> MASSNVTL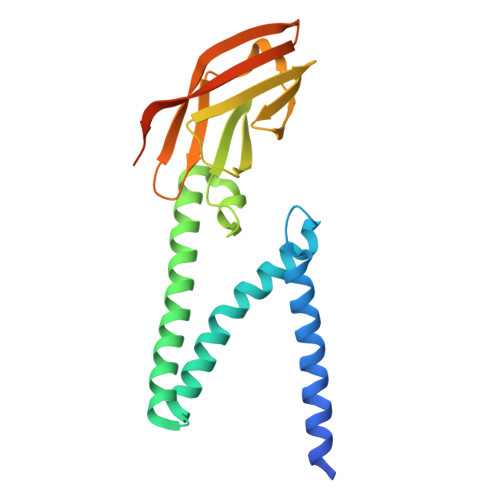SNDEVLRLVKDWNFTWSVVFLLITIVLQYGYPSRSMFVYVIKMFVLWLLWPASMALSIFCAVYPIDLASQIISGILAATSCAMWISYFVQSIRLFMRTGSWWSFNPESNCLLNVPIGGTTVVRPLVEDSTSVTAVVTDGYLKMAGMHFGACDFQRLPSEVTVAKPNVLIALKMIKRQAYGTNSGVAIYHRYKAGNYRRPPIIQDQELALLRA> MNKNLAILTPIVLLSLVLAPIAISAVTINGITFYSPVPNQTYKYGQQLVLSIQSQPNALVTLYVYDPKGNVVYNNVYQTNSSGGLTATIATFGSTPGFTTVGTYTVSLSVQGTTSESASVNVQYVPLTSTITATVVNQEGSPLAGATVQLYNTTSGSNTLVATQTTNSQGVATFTVLSFPGVTQTFKLVASLQGYAASTASVSITGQQNASVTITLVPAVVTIAPMYVIQNGTVIGSGPSLSSIVVYQGLPAYILAQVSFAGQRVTTAPVSAQVYYPNGTQTVKASVITSGKYAGMYNITIMPPTESVQNYVF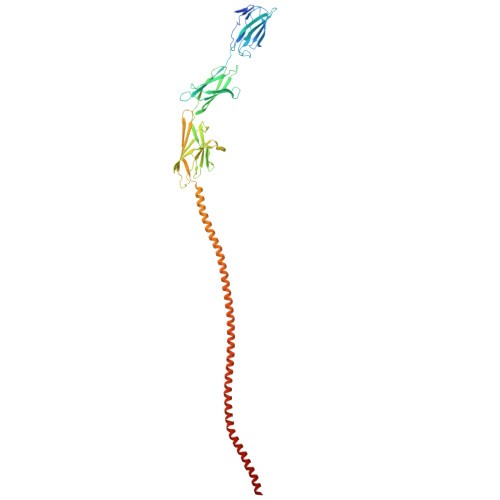QLLIVANYTTSSGQTLSTKYLMSVQANQNLQALVNKEISSLVQNITNLEKTVNNLQTQISTLNSSLSSLSQRITSLQNTLASLNSTISSLSGTASSLSSQLNALQGKISSLNSSITNLSGQLNSLQSKVNSLTPLVYGGIIAGIIGLIVAIVAIVLVYRKIS Multi-subunit SMC complexes control chromosome superstructure and promote chromosome disjunction, conceivably by actively translocating along DNA double helices. SMC subunits comprise an ABC ATPase “head” and a “hinge” dimerization domain connected by a 49 nm coiled-coil “arm. The heads undergo ATP-dependent engagement and disengagement to drive SMC action on the chromosome. Here, we elucidate the architecture of prokaryotic Smc dimers by high-throughput cysteine cross-linking and crystallography.

To do so, we first determined the structure of the upper region of the Py Smc coiled coil, designated as PySmcCC3, comprising residues 345–468 and 694–814 connected via a SGGS linker. The structure refined to 2 Å resolution showed that, while the N-terminal α helix is continuous, the C-terminal helix contains a short non-helical region. This region (residues 774–779) exhibits barely traceable electron densities, and the opposing portion of the N-terminal helix displays better, but weak, electron densities. Helical wheel analysis and sequence alignment indicate that the non-helical region in Py Smc arises from a 2 aa deletion in comparison with other Smc protein, e.g., Bs Smc, which completes a heptad repeat in this region (right). In addition, the N-terminal helix bends noticeably at residue P434, which is unlikely to bear functional importance since P434 is not a conserved residue.

> TKGAIVRWGKRKEKLIEEIRAREEERNALVVRLGEIDRTFAVAREEFDTVVKELEEARKSLYEGEARIKRAEEEKERLKAEILTGEARLPGLRERAENLRRLVEEKRAEISELERRLSSITSKRSGGSLESQSFELRIKLSDLEKELELARKDLEKVLAEERAVREEIEVAKRRINELDTLIERERGELAKLRGRIERLERKRDKLKKALENPEARELTEKIRAVEKEIAALREELSRVEGKLEGLESKVDAGSSSRPGL N-{(1S,2S)-2-[bis(carboxymethyl)amino]cyclohexyl}-N-{(2R)-2-[bis(carboxymethyl)amino]-3-[4-({[2-hydroxy-1,1-bis(hydroxymethyl)ethyl]carbamothioyl}amino)phenyl]propyl}glycine | C30 H45 N5 O13 S | 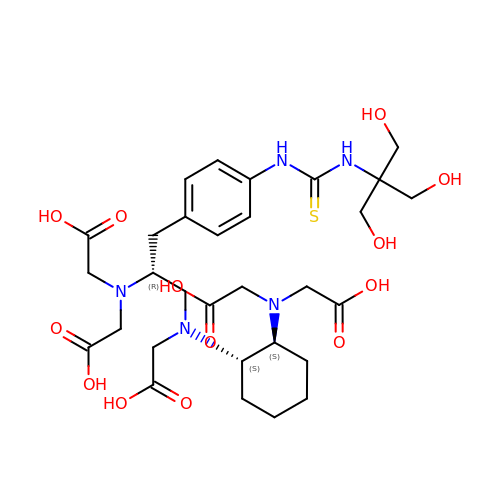ZDJITWBUQUCYMP-VJBWXMMDSA-N> GSHMTATEN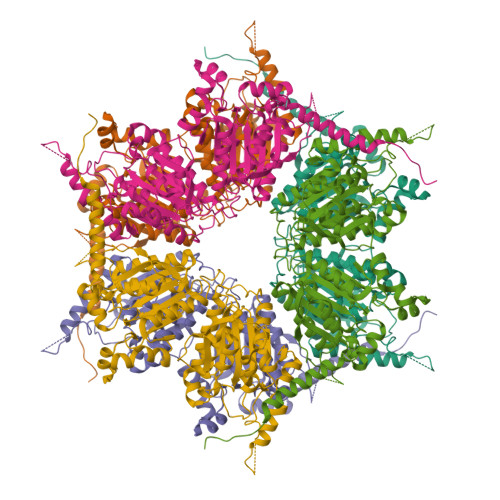ADGRTRRRLDELARRRAELAAQATERGAGRQHAKGKLTARERIDLLLDPDSFTELDALARHRCHNYGMEEQRPYGDGVVTGYGTIDGRKVCVYAQDFTVLGGSLGEVFGEKIIKVLDLAIRTGCPVIGINDSGGARIQEGVVSLAYYAELVKRHVAASGVIPQISLIIGPCAGGAVYAPATTDLVVMVEDISHMFVTGPDVLQAVTGQTVGMEELGGAHRHNAVSGAAHYMAADEKDAFDYVRMVLGHLPSNNMGDTPVFAPTAARELTEADRALDTLIPDRTAESYDMMRVVNAVIDDGELTQFHQLFAPNVICGLARVEGHSVGVVANQPTHLAGALDIDASEKAARFIRFCDAFHVPVLTFVDVPGFLTSMEQERDGIIRRGAKLIYAYCEATVPMVTVITRKAYGGGYGVMGSKHLGIDVNLAWPTAEIAVMGGESAVRIIHRQDIRQAEDPEETRERLVSEYTETMCTPYVAAERGYVDAVIMPHETRAQVATALDTLRDKRMTRLPRKHGNIPL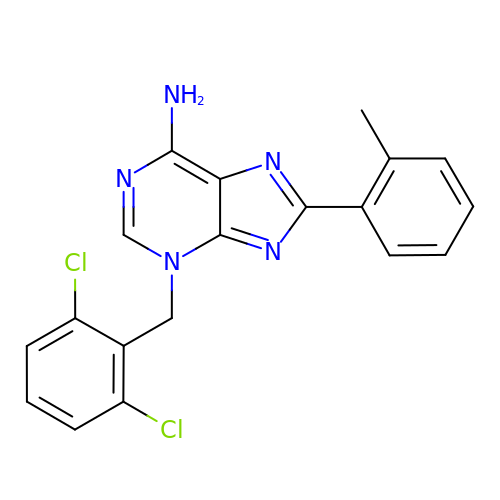3-[(2,6-dichlorophenyl)methyl]-8-(2-methylphenyl)-3H-purin-6-amine | C19 H15 Cl2 N5 | OAGNWWLJSOJIFV-UHFFFAOYSA-N>[4x]SNAMTQEIEIEFKNIVTEEEFHALCKSFSIEVFTKQVNHYFETPNSSLKEAGSALRIR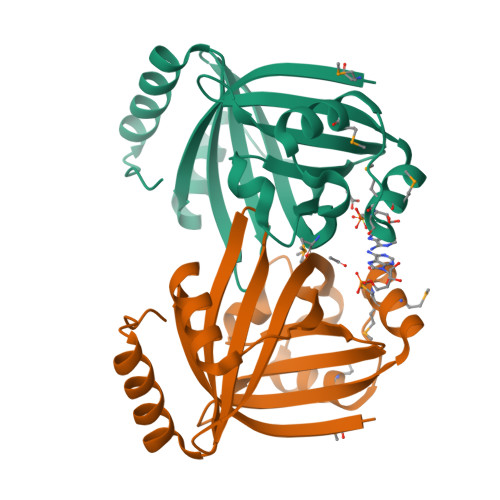HKGETYTLTLKQPAEVGLLETHQVVTENEAKMMMETNVIISGAVMNQLCKLQIPVSALTYMGSLTTERAETLFEGGTLVFDHSFYYNHDDYEIEFEVQDEETGKAAFIHLLKQHNIPIRHTNNKVKRFFLAKQNKAR2-amino-7-(pyridin-3-ylmethyl)-3,5-dihydro-4H-pyrrolo[3,2-d]pyrimidin-4-one | C12 H11 N5 O | 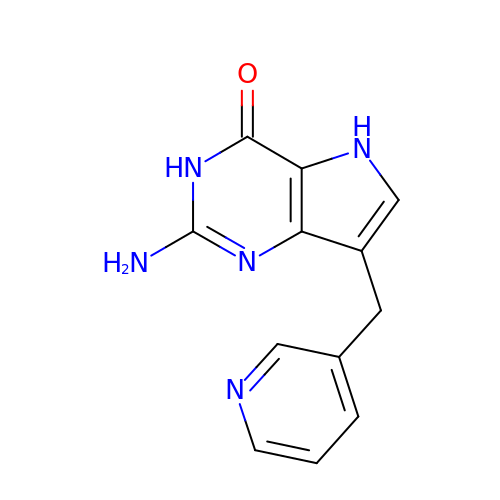DOHVAKFYAHLCJP-UHFFFAOYSA-N> MAPIEYLLFEEPTGY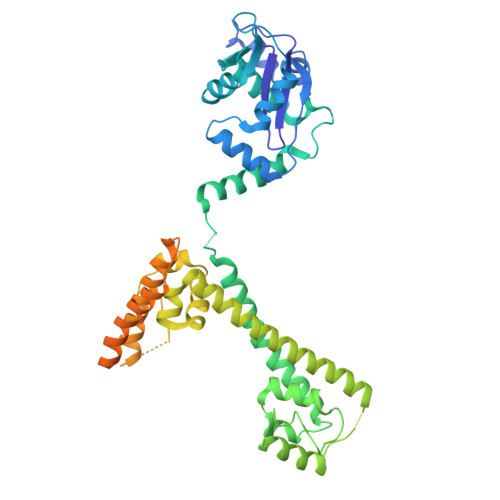AVFKVKLQQDDIGSRLKEVQEQINDFGAFTKLIELVSFAPFKGAAEALENANDISEGLVSESLKAILDLNLPKASSKKKNITLAISDKNLGPSIKEEFPYVDCISNELAQDLIRGVRLHGEKLFKGLQSGDLERAQLGLGHAYSRAKVKFSVQKNDNHIIQAIALLDQLDKDINTFAMRVKEWYGWHFPELAKLVPDNYTFAKLVLFIKDKAXXXXXXXXXXXXXXXXXXXXXXXXXXSETDMENVCVFAQRVASLADYRRQLYDYLCEKMHTVAPNLSELIGEVIGARLISHAGSLTNLSKQAASTVQILGAEKALFRALKTKGNTPKYGLIYHSGFISKASAKNKGRISRYLANKCSMASRIDNYSEEPSNVFGSVLKKQVEQRLEFYNTGKPTLKNELAIQEAMELYNKDKPAAEVEETKEKESSKKRKLEDDDEEKKEKKEKKSKKEKKEKKEKKDKKEKKDKKEKKDKKKKSKD(2~{R},3~{R})-4,4-bis(fluoranyl)-2-(hydroxymethyl)oxolan-3-ol 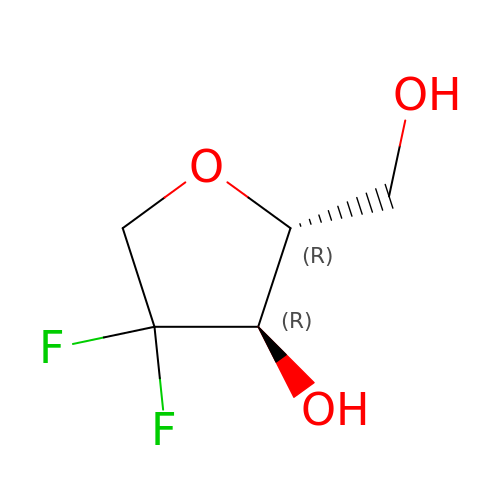| C5 H8 F2 O3 | XLFTWOXMFCMHBS-QWWZWVQMSA-N>HHHHHHFNLPPGNYKKPKLLYCSNGGHFLRILPAGTVDGTRDRSDQHIQLQLSAESVGEVYIKSTETGQYLAMDTDGLLYGSQTPNEECLFLERLEENHYNTYISKKHAEKNWFVGLKKNGSCKRGPRTHYGQKAILFLP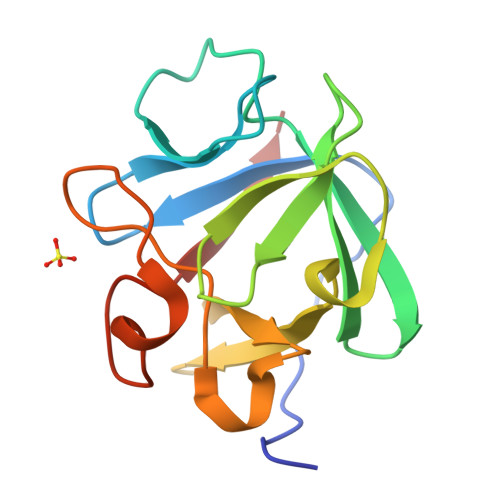LPVSSD[2x]>[2x]HHHHHHSDEALKMTMASVPASRYLTDMTLEEMSRDWSMLIPK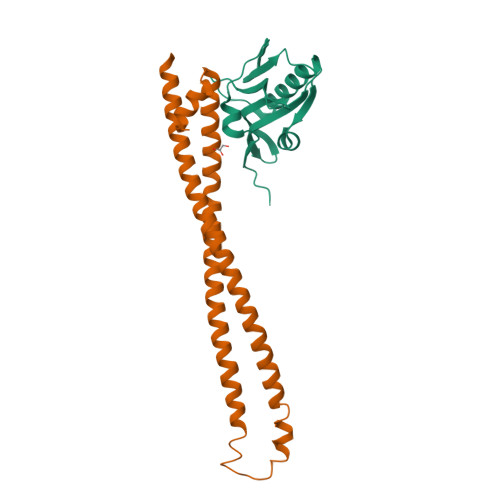QKVAGPLCIRMDQAIMDKNIILKANFSVIFDRLETLILLRAFTEEGAIVGEISPLPSLPGHTAEDVKNAVGVLIGGLEWNDNTVRVSETLQRFAWRSSNENGRPPLTPKQKREMAGTIRSEV;>YQQDQIVKEDSVEAVGAQLKVYHQQYQDKSREYDQLYEEYTRTSQELQMKRTAIEAFNETIKIFEEQGQTQEKSSKEYLERFRREGNEKEMQRILLNSERLKSRIAEIHESRTKLEQELRAQASDNREIDKRMNSLKPDLMQLRKIRDQYLVWLTQKGARQKKINEWLGI[2x]(7S,10S,13S)-10-(4-aminobutyl)-7-(3-aminopropyl)-17,20-dichloro-13-[(1H-indol-3-yl)methyl]-12-methyl-6,7,9,10,12,13,15,16-octahydropyrido[2,3-b][1,5,8,11,14]benzothiatetraazacycloheptadecine-8,11,14(5H)-trione 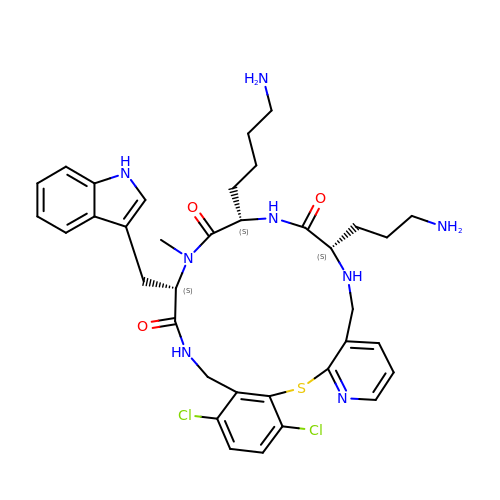| C36 H44 Cl2 N8 O3 S | GBONSZKSVKTWGU-CHQNGUEUSA-N>[3x]MATEGMILTNHDHQIRVGVLTVSDSCFRNLAEDRSGINLKDLVQDPSLLGGTISAYKIVPDEIEEIKETLIDWCDEKELNLILTTGGTGFAPRDVTPEATKEVIEREAPGMALAML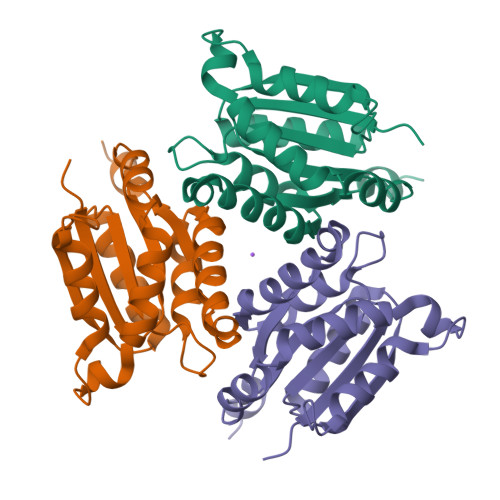MGSLNVTPLGMLSRPVCGIRGKTLIINLPGSKKGSQECFQFILPALPHAIDLLRDAIVKVKEVHDRSHHHHHH> MVVLDKKLLERLTSRKTPLEELEDMEKRCFLSTFTYQDAFDLGTYIRNAVKENFPEKPVAIDISLPNGHCLFRTVTYGGSALDN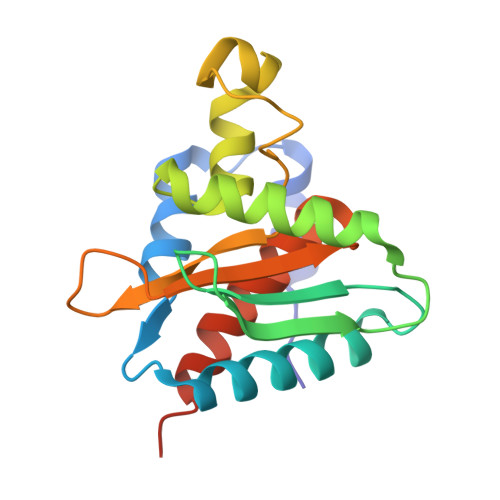DFWIQRKKKTALRFGHSSFYMGCKKGDKTPEEKFFVDSKEYAFHGGAVLIQSERSDYPYACLTISGLKQEEDHLMAVSSLIAFANESLEEDLNLD>[2x]SMKNRLWVSNKAQTTAADKAPLFDFSAGECRFYKTLSDSEYYVKDHVVHEKTVLPGAAIIEAAREAGERLYGKSVIKLSQVVWAVPITVEKEKTIM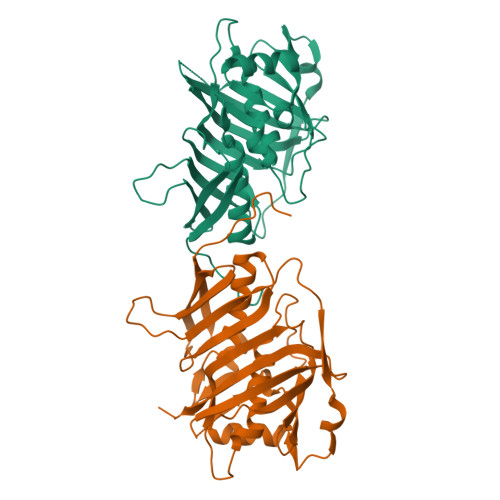IDLLPNQKDGRFVVKTDMQPEAAVHCQGNIITCGDQDASHTERFQLDSWLTGQKRLISSAECYRDFRQSGLEYGASFQVIKQLFIHENAVLARISLPESIHKKSGTLLEPCLLDGIFQSTTGFTSGQEDDHTAYLPFELGELEILHAPSANGYAYITAADERQHDDVKRFHILFMDENGSVSLKIKNLALKALRAAPQTQDERHSVK> LPLNSDYSLLLTFIYGGRVVGKTQVHSLDCRLVAERSDSESSMEQVEFPKPDPLEPTQHLLNQLDRGVLVASNSRGLFVQRLCPIPISWNAPEAPPGPGPHLLPSNKCVELFKTTYFCRDLAQYFQG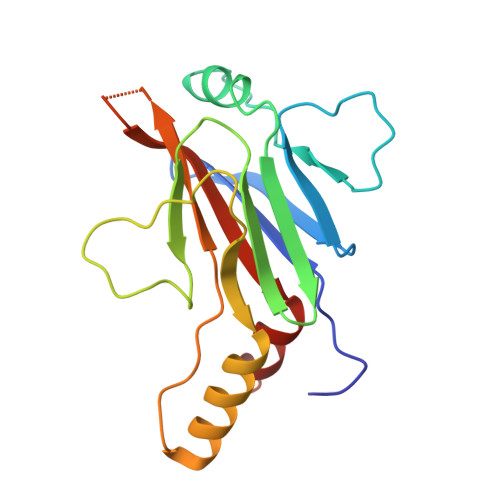QGPPPKFQATLHFWAASPGSSHSQENLITVQMEQAFARHLLEKI3-amino-5-[(4-chlorophenyl)amino]-N-[(1S)-1-phenylethyl]-1H-1,2,4-triazole-1-carboxamide 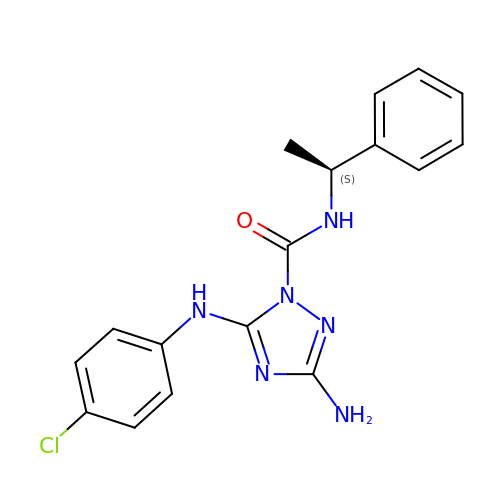| C17 H17 Cl N6 O | ZLOKMYYNNUNJBU-NSHDSACASA-N>[4x]MDKFRVQGPTRLQGEVTISGAKNAALPILFAALLAEEPVEIQNVPKLKDIDTTMKLLTQLGTKVERDGSVWIDASNVNNFSAPYDLVKTMRASIWALGPLVARFGQGQVSL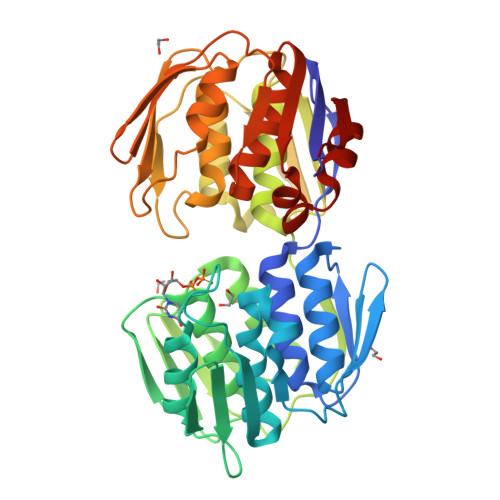PGGDAIGARPVDLHIFGLEKLGAEIKLEEGYVKASVNGRLKGAHIVMDKVSVGATVTIMSAATLAEGTTIIENAAREPEIVDTANFLVALGAKISGQGTDRITIEGVERLGGGVYRVLPDRIETGTFLVAAAISGGKIVCRNAQPDTLDAVLAKLREAGADIETGEDWISLDMHGKRPKAVTVRTAPHPAFPTDMQAQFTLLNLVAEGTGVITETIFENRFMHVPELIRMGAHAEIESNTVICHGVEKLSGAQVMATDLRASASLVLAGCIAEGTTVVDRIYHIDRGYERIEDKLRALGANIERVKGE> TPVPSTGNPFEGYDIYLSPYYAEEVEAAAAMIDDPVLKAKALKVKEIPTFIWFDVVRKTPDLGRYLADATAIQQRTGRKQLVQIVVYDLPDRACAAAASNGEFSLADGGMEKYKD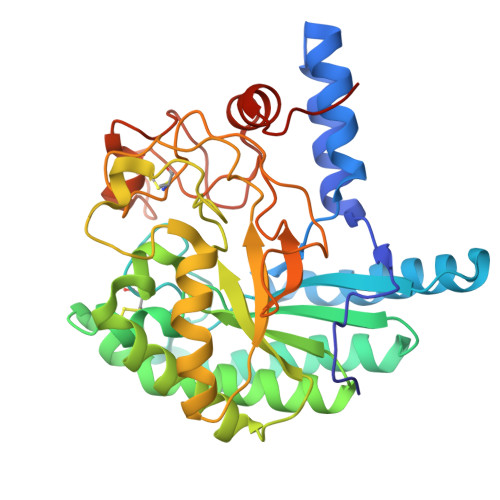YVDRLASEIRKYPDVRIVAVIEPDSLANMVTNMNVAKCRGAEAAYKEGVIYALRQLSALGVYSYVDAGHAGWLGWNANLAPSARLFAQIYKDAGRSAFIRGLATNVSNYNALSATTRDPVTQGNDNYDELRFINALAPLLRNEGWDAKFIVDQGRSGVQNIRQEWGNWCNVYGAGFGMRPTLNTPSSAIDAIVWIKPGGEADGTSDTSAPRYDTHCGKSDSHKPAPEAGTWFQEYFVNLVKNANPPLAAALEHHHHHH>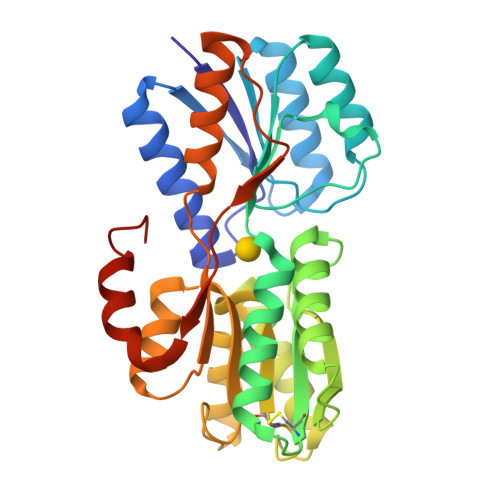 APLTVGFSQVGSESGWRAAETNVAKSEAEKRGITLKIADGQQKQENQIKAVRSFVAQGVDAIFIAPVVATGWEPVLKEAKDAEIPVFLLDRSIDVKDKSLYMTTVTADNILEGKLIGDWLVKEVNGKPCNVVELQGTVGASVAIDRKKGFAEAIKNAPNIKIIRSQSGDFTRSKGKEVMESFIKAENNGKNICMVYAHNDDMVIGAIQAIKEAGLKPGKDILTGSIDGVPDIYKAMMDGEANASVELTPNMAGPAFDALEKYKKDGTMPEKLTLTKSTLYLPDTAKEELEKKKNMGYLEHHHHHHH> MALLRALA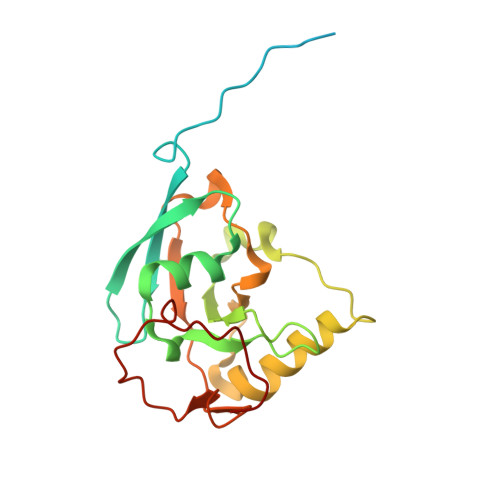KPLRSLQAVSSVAQVSLRQFGAASHHDDHHDDHDHYTPPKTVFEDTITINVLDYDGKKHAVKALIGTPLNKALVEYGFSSTYFFPNMGYYTQHISDAHVFIPEEYWKYVENVDLKTDDAEAIKLMFKLVVQDYQRETSFFASYLTLNKEMDNMTIGFGPIKPWHITPKWSFNGHHNVKDRMFDRLETGPFIE> KIIHLTDDSFDTDV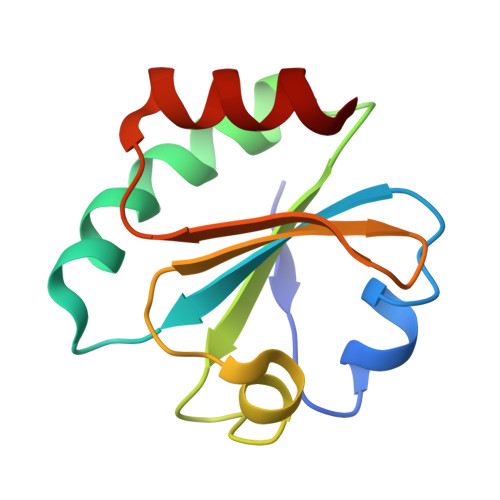LKADGAILVDFWAEWCGPCKMIAPILDEIADEYQGKLTVAKLNIDQNPGTAPKYGIRGIPTLLLFKNGEVAATKVGALSKGQLKEFLDANL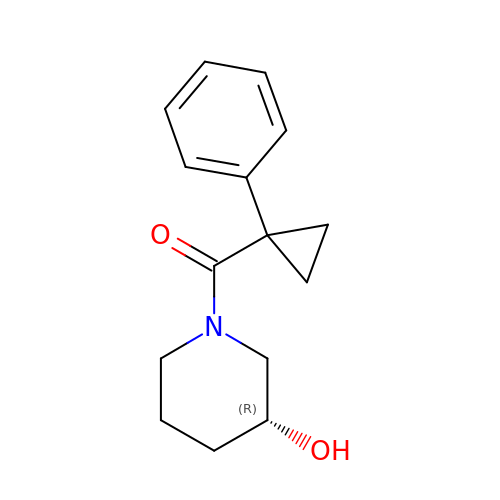[(3R)-3-hydroxypiperidin-1-yl](1-phenylcyclopropyl)methanone | C15 H19 N O2 | NMEGOWUYSINAGN-CYBMUJFWSA-N> MLRFTHRALTATPERFSVLGTTHPKPKRTGFGRNNKMRSKPSDNVAWYDKGPVEWLPRPVRLTYDHLDQLQQWTM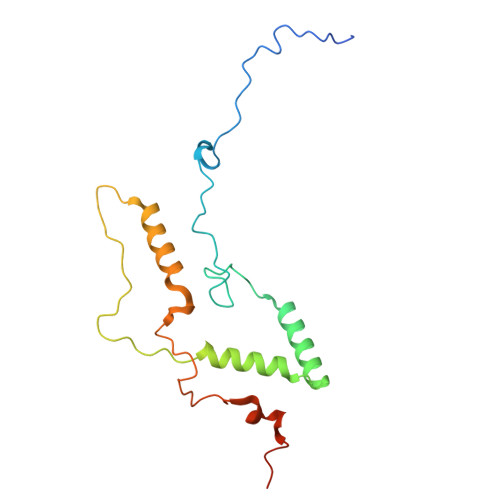RATLDGRTEEFNRIRDLHREWSQHPLMPVLGDVEPKFPLNLFKQNHRAKKRFLVRWHKANTPANWLWMPRGPTVVTPLHRTNPTQYPENWKQMVQRKSGTGTPS> AESKPTPQSTFTGPIVVDPITRIEGHLRIMVEVENGKVKDAWSSSQLFRGLEIILKGRDPRDAQHFTQRACGVCTYVHALASSRCVDDAVKVSIPANARMMRNLVMASQYLHDHLVHFYHLHALDWVDVTAALKADPNKAAKLAASIAPARPGNSAKALKAVQDKLKAFVESGQLGIFTNAYFLGGHKAYYLPPEVDLIATAHYLEALHMQVKAASAMAILGGKNPHTQFTVVGGCSNYQGLTKDPLANYLALSKEVCQFVNECYIPDLLAVAGFYKDWGGIGGTSNYLAFGEFATDDSSPEKHLATSQFPSGVITGRDLGKVDNVDLGAIYEDVKYSWYAPGGDGKHPYDGVTDPKYTKLDDKDHYSWMKAPRYKGKAMEVGPLARTFIAYAKGQPDFKKVVDMVLGKLSVPATALHSTLGRTAARGIETAIVCANMEKWIKEMADSGAKDNTLCAKWEMPEESKGVGLADA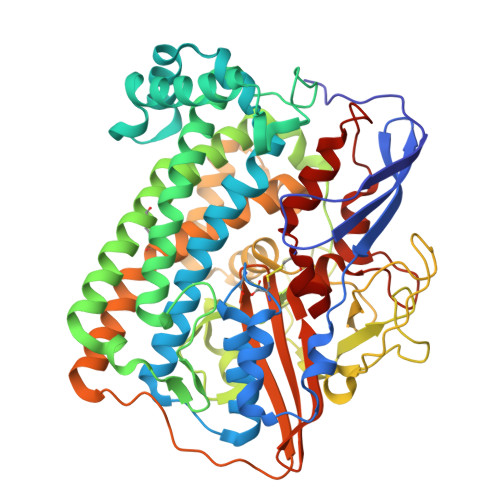PRGALSHWIRIKGKKIDNFQLVVPCTWNLGPRGAQGDKSPVEEALIGTPIADPKRPVEILRTVHAFDPCIACGVH>MKFGIEFVPNEPIQKLCYYVKLAEDNGFEYCWITDHYNNRNVYMALTAIAMNTNKIKLGPGVTNPYVRSPA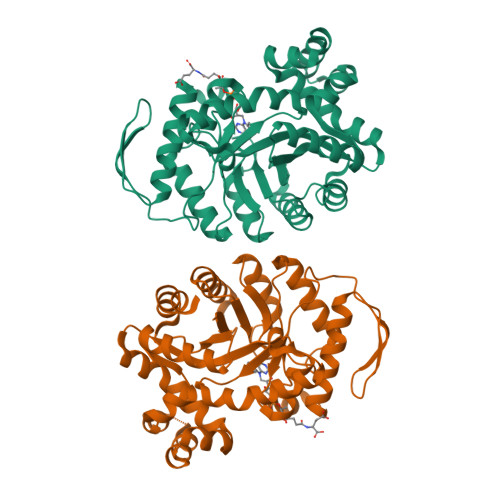ITASAIATLDELSGGRAVLGIGPGDKATFDALGIEWVKPVTTLKESIEVIRKLLAGERVSYEGKVVKIAGAALAVKPIQKAVPVYMGAQGPKMLETAGMIADGVLINASNPKDFEAAIPLIKKGAEAAGRSMDEIDVAAYACMSVDKNADKAKQAAVPVVAFIAAGSPPVVLERHGIDMEKVEAIRNALKSGNFPEAFKNVDDTMLEAFSIYGTPEDVVEKCKKLAEMGVTQIVAGSPIGPNKETAIKLIGKKVIPALKE[2x]>[2x]GSHMASMREFIFKANKTITSSDINLKDLPGSCGRLDLLCRCVS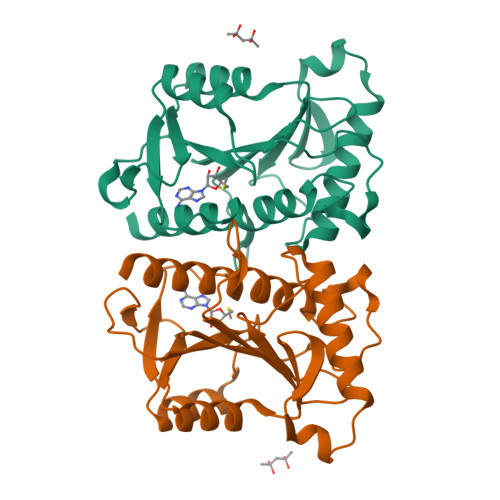DAFFLSHDIRRDVVFYAVLYGQPNPPVCIKFVGSELKKVSPDERNIAIFIKKALKKFEELDEEQRKDWNQSTPGIYVRRLGFRNLVLEKLEEGKNIYYLHMNGEDVENVDIENPVFIIGDHIGIGEEDERFLDEIKAKRISLSPLELHANHCITIIHNVLDKKRICEI>MAHHHHHHVDDDDKMVHHDGFQTVKATIDWEHPMFKLYEKAKRNGKWNPADIDFSQDQKDFASLTSEEKISALPLVAGFSAGDEAVTLDILPMAHALARQGRLEDVLFLTTFMHDEAKHVEMFSRWQQAVGIGQMDLSVFHNDHYKRIFYEALPEAMNRLYADDSPEAVIRAATVYNMIVEGTLAESGYYTFRQIYKKAGLFPGLLQGIDYLNMDEGRHIQFGIYTIQRIVNEDERYYELFIRYMDELWPHVIGYVDYLTELGKRQQQLARTYALEID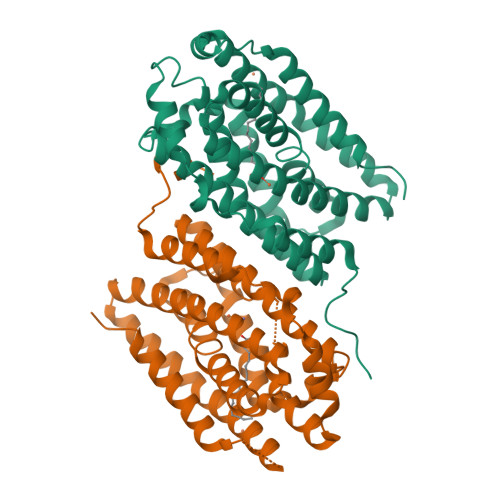YDLLRHYVIKQFNLRKKQISRTKRVDVVEGLEKTAAES[2x]> MELTLGLVAIASAILIAFGALGTAIGFGLLGGRFLEAVARQPELAPQL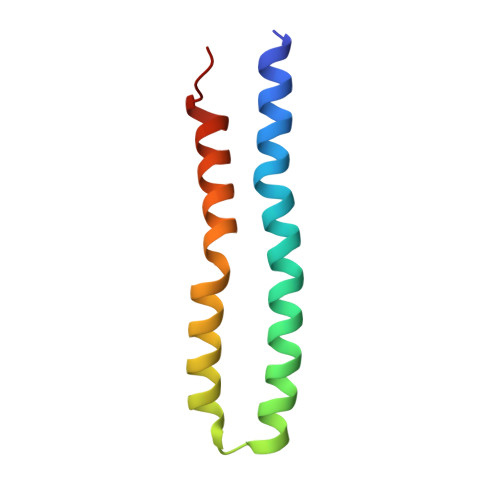QTRMFLIAGLLDAVPMIGVGIGLFFIFANPFVG>MIRFEHVSKAYLGGRQALQGVTFHMQPGEMAFLTGHSGAGKSTLLKLICGIERPSAGKIWFSGHDITRLKNREVPFLRRQIGMIFQDHHLLMDRTVYDNVAIPLIIAGASGDDIRRRVSAALDKVGLLDKAKNFPIQLSGGEQQRVGIARAVVNKPAVLLADQPTGNLDDALSEGILRLFEEFNRVGVTVLMATHDINLISRRSYRMLTLSDGHLHGGVGHE[2x];>MNKRDAINHIRQFGGRLDRFRKSVGGSGDGGRNAPKRAKSSPKPVNRKTNVFNEQVRYAFHGALQDLKSKPFATFLTVMVIAISLTLPSVCYMVYKNVNQAATQYYPSPQITVYLQKTLDDDAAAGVVAQLQAEQGVEKVNYLSREDALGEFRNWSGFGGALDMLEENPLPAVAVVIPKLDFQGTESLNTLRDRITQINGIDEVRMDDSWFARLAALTGLVGRVSAMIGVLMVAAVFLVIGNSVRLSIFARRDSINVQKLIGATDGFILRPFLYGGALLGFSGALLSLILSEILVLRLSSAVAEVAQVFGTKFDINGLSFDECLLLLLVCSMIGWVAAWLATVQHLRHFTPE[2x];> MTRAVKPRRFAIRPIIYASVLSAGVLLCAFSAHADERDQLKSIQADIAAKERAVRQKQQQRASLLAQLKKQEEAISEATRKLRETQNTLNQLNKQIDEMNASIAKLEQQKAAQERSLAAQLDAAFRQGEHTGIQLILSGEESQRGQRLQAYFGYLNQARQETIAQLKQTREEVAMQRAELEEKQSEQQTLLYEQRAQQAKLTQALNERKKTLAGLESSIQQGQQQLSELRANESRLRNSIARAEAAAKARAEREAREAQAVRDRQKEATRKGTTYKPTESEKSLMSRTGGLGAPRGQAFWPVRGPTLHRYGEQLQGELRWKGMVIGASEGTEVKAIADGRVILADWLQGYGLVVVVEHGKGDMSLYGYNQSALVSVGSQVRAGQPIALVGSSGGQGRPSLYFEIRRQGQAVNPQPWLGR

FtsEX, an important component of the divisome, is mainly recognized for its involvement in activating the degradation of sPG through amidases via the periplasmic factor EnvC. FtsEX belongs to the Type VII ABC superfamily, which includes LolCDE and MacB. In contrast to the reported ABC transporters, FtsEX neither transports anything across the membrane nor extracts substances from the membrane but interacts with EnvC to form the sPG hydrolysis machinery to separate the daughter cells during cell division. The activation of AmiA and AmiB by EnvC is controlled by the cell division protein complex FtsEX, which induces conformational changes in EnvC through ATP hydrolysis.

Consequently, the structure of the complete FtsEE163QX-EnvC complex consists of 2 copies of FtsE, 2 copies of FtsX, and a single EnvC. Based on the cryo-EM map of FtsEX-EnvC, we built a model incorporating FtsE, FtsX, and EnvC coiled-coil domain. The core domains, including the transmembrane and nucleotide binding domains, are determined at 2.8 Å, while the periplasmic domains of FtsX are determined at 3.8 to 4.5 Å. Notably, the cryo-EM map of the restraining arm and LytM domain of EnvC are almost invisible. We observed that in the ATP-bound FtsEE163QX-EnvC complex structure, the 2 copies of FtsX appeared to be asymmetric. According to the superimposition of the 2 FtsX from the FtsEX-EnvC complex, the transmembrane helices of the 2 FtsX molecules are almost identical in conformation, but the periplasmic domain of one FtsX, compared to the other, shifts approximately 17.5 Å and rotates 37°. We speculate that the binding of EnvC results in a relatively rigid conformation of the FtsX periplasm domain, while the transmembrane domain of FtsX is almost identical. The 2 X-lobe structures of FtsX tightly bound to the CC domain, which couples the conformational changes between FtsX and EnvC. When our structure ecFtsEE163QX-EnvC(ATP) and the paFtsEX-EnvC(apo), paFtsEX-EnvC(ATP) structures are superimposed using one FtsE as a reference, we observe overall similarity between our ecFtsEE163QX-EnvC(ATP) and the paFtsEX-EnvC(apo) structures, with conformational differences are observed on the EnvC coiled-coil domain. Furthermore, it was found that FtsEE163QX-EnvC (ATP) had a similar effect to FtsEX-EnvC (AMP-PNP). These findings suggest that FtsX-EnvC, like EnvC, only moderately activates AmiB, while ATP-bound FtsEE163QX-EnvC strongly enhances AmiB activity.>PVEEVMPVLEEKERSASYKPVFVTEITDDLHFYVQDVETGTQFQKLMENMRNDIASHPPVEGSYAPRRGEFCIAKFVDGEWYRARVEKVESPAKIHVFYIDYGNREVLPSTRLGTLSPAFSTRVLPAQATEYAFAFIQVPQDDDARTDAVDSVVRDIQNTQCLLNVEHLSAGCPHVTLQFADSKGDVGLGLVKEGLVMVEVRKEKQFQKVITEYLNAQESAKSARLNLWRYGDFRADDADEFGY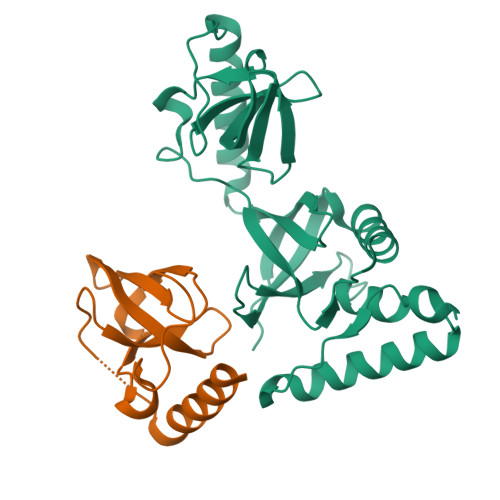SR[2x]[(4-{2-[(3-hydroxyphenyl)amino]-1H-benzimidazol-1-yl}-1,3,5-triazin-2-yl)amino]acetonitrile | C18 H14 N8 O | 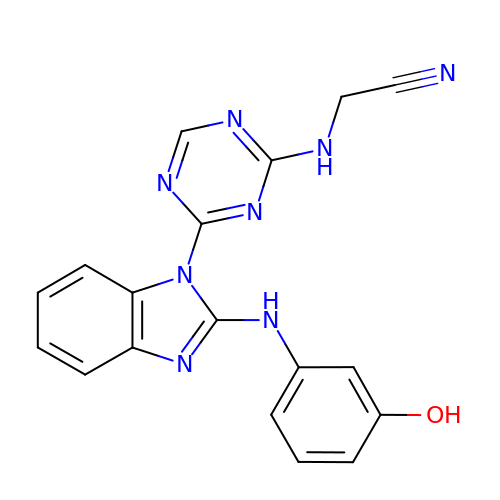FEBJYEFFVIDUNF-UHFFFAOYSA-N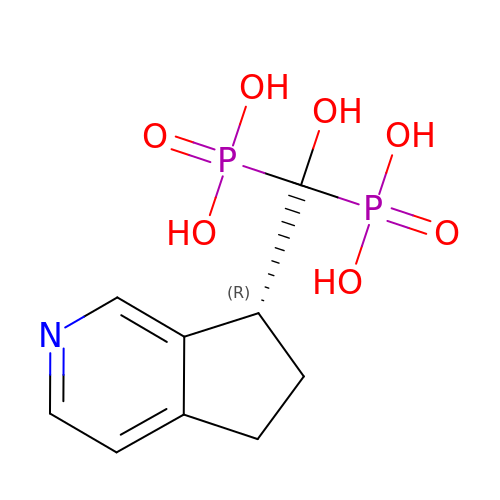[(7R)-6,7-dihydro-5H-cyclopenta[c]pyridin-7-yl(hydroxy)methylene]bis(phosphonic acid) | C9 H13 N O7 P2 | WBALRBOBYFLYPZ-MRVPVSSYSA-N>KDRPSLCDLPADSGSGTKAEKRIYYNSARKQCLRFDYTGQGGNEN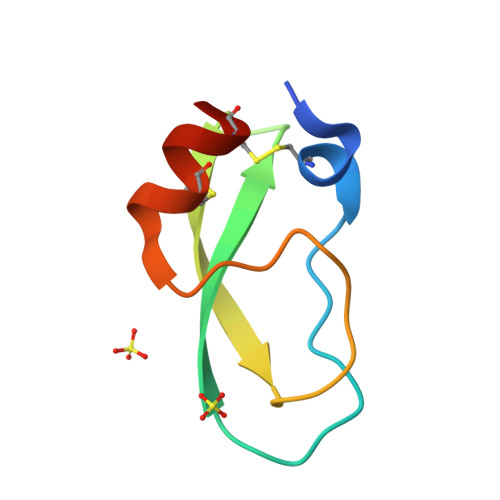NFRRTYDCQRTCLYT[6x]>[2x]SMEEEIEEAYDLVEEAEKTGDTSLLKKAKELLDKVAEEATKSGNPILLIRVIIILIKIVRNSGDPSVAALARELLEKLEEIAEKEGNRFIEAMGEALRTQIERAL

We reasoned that to enable systematic design of binders to convex protein target sites it would be necessary to generate scaffold sets with overall concave shapes. We focused on 5 helix bundle scaffolds with three helices forming the concave interface and two helices providing structural support. The selected 7476 scaffolds, which we refer to as 5HCS (5 helix concave scaffolds) throughout the remainder of the text, have a wide range of curvatures. Our method for computationally designing small but concave proteins to bind to convex protein target sites expands the space of the protein surfaces that can be targeted by de novo protein design.

Programmed death-ligand 1 (PD-L1), is upregulated on many tumors, and interacts with PD-1 on T-cells to downregulate T-cell activation. We optimized the stronger binder, 5HCS_PDL1_0, by resampling the residues at the designed interface using ProteinMPNN15 followed by Alphafold28 filtering. The highest affinity binder, 5HCS_PDL1_1, which has 93.2% similarity with the sequence of 5HCS_PDL1_0, is expressed at high levels, very stable and has an affinity of 646 pM. We solved the high resolution crystal structure of 5HCS_PDL1_1. The refined structure has excellent geometry and reveals the expected helical assembly with five antiparallel helices. The crystal structure of 5HCS_PDL1_1 superimposes on the computational design model with a rmsd of 0.75 Å over 105 aligned Cα atoms (the substitutions which increase affinity relative to 5HCS_PDL1_0 do not alter the backbone structure). As with 5HCS_TGFBR2_1 and 5HCS_CTLA4_1, the interfacial helices H1, H3 and H5 of 5HCS_PDL1_1 have an overall concave shape. The key interactions between H1 and PD-L1 include aromatic packing of Y9 and Y123 on PD-L1 and electrostatic interactions between D10 and E13 with K124 and R125 on PD-L1. H3 binds to the hydrophobic pocket formed by Y56, M115, A121 and Y123. Residues Y9, E13, K56 and Q99 spanning the three helices satisfy the hydrogen bonding requirements of both the side chains and backbone of the PD-L1 edge beta strand (A121-R125) buried at the interface.>[5x]MATEQIQHIAIVGCVHGKYREMYRQLSEYEKSTGKEISFVICTGDMQTLRYEADLVYLKVPPKYKQMGDFHLYYEGKEKAPYLTLFIGGNAESSNVLLHLYNGGFVCFNMYYLGVCSCININGLRIVGVSGIYKSFDEKKPYTYPPSPNDVVSLFHTRNYVIQMLSN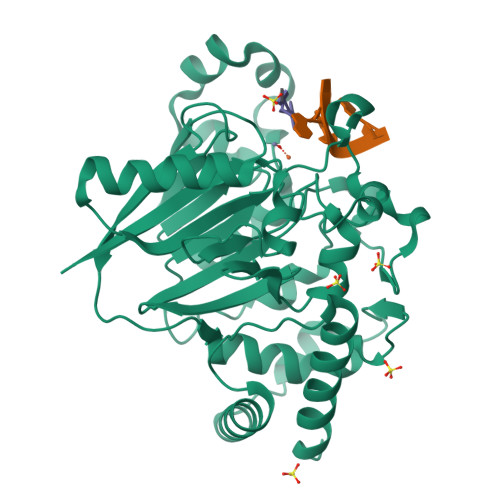LSQSSQIDISLSHDWPQGIVMKGNYKQLYRFQPGFKKDGASLGSPINKVILNTLKPKYWISGHMHCEYHAEEGPTHFIALGKIGYKNAISYLDLPLKQKTDLEYDKDWVCNLIMTWPAFSNKAQFPDLSYSISELLSKRTKELDKKIIELWEKYIGLKIIYDSDTFDIQFTSRRFYIEKIYNELNINHHHHHH DnaJ protects the cell from adverse conditions through the prevention of protein aggregation or by assisting the refolding of unfolded proteins and is an essential partner of the chaperone DnaK in bacterial DnaK–DnaJ–GrpE chaperone systems. DnaJ, the bacterial homologue of Hsp40, stimulates ATP hydrolysis by DnaK (Hsp70) and thus mediates capture of substrate protein, but is also known to possess chaperone activity of its own. T. thermophilus DnaJ is a typical type II DnaJ, i.e. it lacks the zinc-finger domains found in type I DnaJs such as that of E. coli. Crystal structures of the complete molecular cochaperone DnaJ from Thermus thermophilus comprising the J, GF and C-terminal domains and of the J and GF domains alone showed an ordered GF domain interacting with the J domain.

Based on limited proteolysis of a DnaK–DnaJ–DafA complex, we first designed a construct containing the first 114 amino acids (DnaJ114), comprising the J and GF domains, and determined its structure to 1.64 Å resolution by radiation-damage-induced phasing from a mercury(II) chloride derivative. After the Pro6 motif, the GF domain folds onto one side of the J domain in a spiral, making extensive hydrophobic interactions, mainly via the conserved phenylalanine residues. Only two hydrogen bonds are formed between the J and the GF domains: from the Tyr69 hydroxyl group to the side chain of Glu99 and between the side chains of Glu52 and Ser94. In correspondence with the NMR observations for the partially disordered E. coli DnaJ GF domain, the T. thermophilus DnaJ GF domain binds to helix III of the J domain opposite helix II. The same interaction is seen in all six independent copies of the J/GF domains in the DnaJ114 structure. In the DnaJ114 structure, no electron density was observed for residues 108–114 connecting the GF and the C-terminal domains in the complete protein.

>[6x]AAKKDYYAILGVPRNATQEEIKRAYKRLARQYHPDVNKSPEAEEKFKEINEAYAVLSDPEKRRIYDTYGTTEAPPPPPPGGYDFSGFDVEDFSEFFQELFGPGLFGGFGRRSR N-(3-carboxypropanoyl)-L-valyl-N-{(1R)-1-[(S)-hydroxy(oxido)phosphanyl]-2-phenylethyl}-L-prolinamide | C22 H32 N3 O8 P | 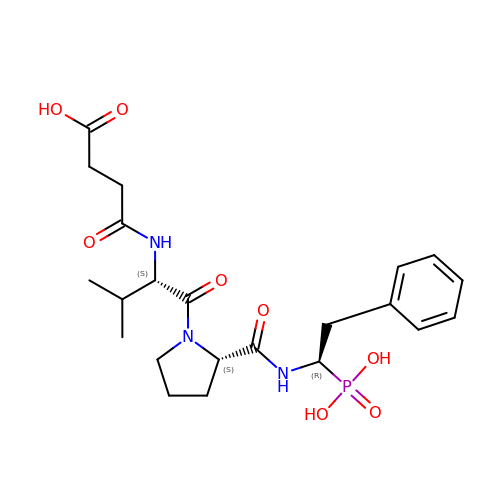KPGFVOVOBVGIMY-HQRMLTQVSA-N>MGLLGSSSSTTPVSKEYKQQLMGSPVYIQIFKEERTLDLYVKMGEQYQLLDSYKICKYSGGLGPKQRQGDFKSPEGFYSVQRNQLKPDSRYYKAINIGFPNAYDRAHGYEGKYLMIHGDCVSIGCYAMTNQGIDEIFQFVTGALVFGQPSVQ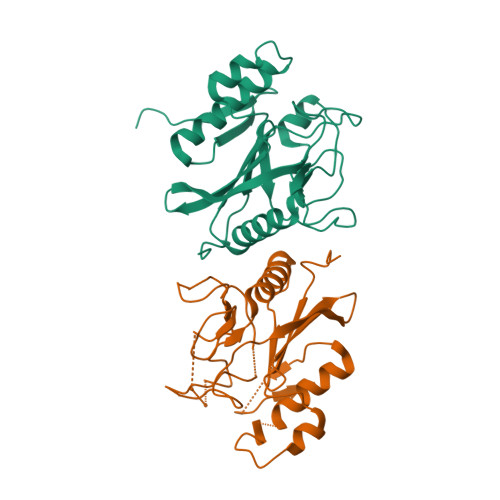VSIYPFRMTDANMKRHKYSNFKDFWEQLKPGYDYFEQTRKPPTVSVVNGRYVVSKPLSHEVVQPQLASNYTLPEAKLEHHHHHH[2x]>[3x]LKVREDENNPFYLRSSNSFQTLFENQNGRIRLLQRFNKRSPQLENLRDYRIVQFQSKPNTILLPHHADADFLLFVLSGRAILTLVNNDDRDSYNLHPGDAQRIPAGTTYYLVNPHDHQNLKIIKLAIPVNKPGRYDDFFLSSTQAQQSYLQGFSHNIL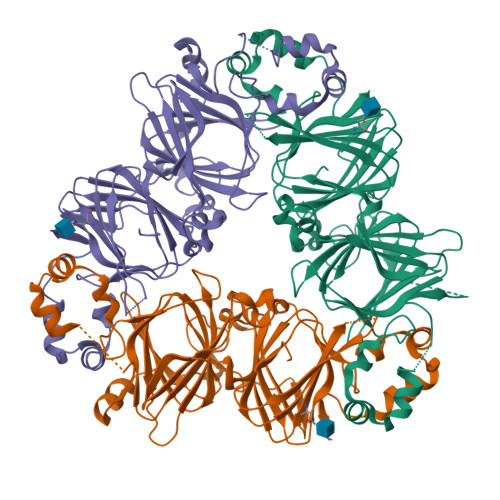ETSFHSEFEEINRVLLGEEEEQRQQEGVIVELSKEQIRQLSRRAKSSSRKTISSEDEPFNLRSRNPIYSNNFGKFFEITPEKNPQLRDLDIFLSSVDINEGALLLPHFNSKAIVILVINEGDANIELVGIKEQQQKQKQEEEPLEVQRYRAELSEDDVFVIPAAYPFVVNATSNLNFLAFGINAENNQRNFLAGEKDNVVRQIERQVQELAFPGSAQDVERLLKKQRESYFVDAQPQQKEEGSKGRKGPFPSILGALY>[2x]MAPSENYTWKNVRIDGGGFVPGIIFNQKEADLIYARTAIGGAYRWNSATSSWIPLLDWVGWDNWGWNGVMSLATDAADPNRVYAAVGMYTNTWDPNNGAILRSTDRGNTWQATPLPFKVGGNMPGRGMGERLAIDPNRNSIIYYGAEGGNGLWRSTDYG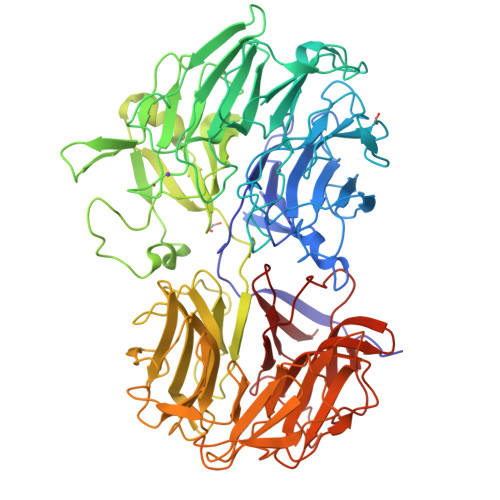ATWAKVSSFTNGGNYAQDPNDPNDYLNKIQGVVWVTFDPASGSAGNTSQVIYVGVADTQNAIYRSTDGGTTWSRLAGQPTGFLPHKGVYDAVNGVLYIAYSDTGGPYDGAKGDVWKFTASSGTWTNISPIPSSSSDLYFGYSGLTIDRKNPNTLMVASQIAWWPDAVFFRSTNGGASWTRIWDWTSYPSRSFRYTMDITEVPWLNFGNSNPVAPEVSPKLGWMNESVEIDPHNSNRLMYGTGATIYATENLTSWDSGGQILLKPMVKGLEETAVLDVVSPPVGAPVYSALGDIGGFRHDDLTKVPTSMYTTPNFSSTTSIDFAELQPATMVRVGNLDSGGGIGVTTNAGGSWWQGQNPPGVTSGGNVALAADGGAIVWAPGGSTNVYLSTTFGSTWTAISALPAGAVIEADRVNPNKFYALANGTFYVSTNKGASFSATVTAGIPAAARKFKAVYGREGDIWLAGGSSTTTYGLWRSTNSGASFTKLASVQEADNVTFGKAATGATYPAIYIIGKVDNVRGVFRSTNEGASWVRINDDQRQYGNFGEAISGDPRIYGRLYLGTNGRGLLYGDSA>MQGLVVSTHPIYLIAKEITKGVEEPQLLLQGQSGHDVQLTPAHRKAINDASLVIWLGKAHEAPLNKLLSNNKKAIALLDSGILSILPQRNTRGAALPNTVDTHVWLEPNNAVRIGFFIAALRSQQHPENKAKYWNNANTFARNMLQAAQAYDSSSNGKPYWSYHDAYQYLERSLNLKFAGALTDDPHVAPTAAQIKYLNDSRPKAQMCLLAESFTTKGQYQKLGSITF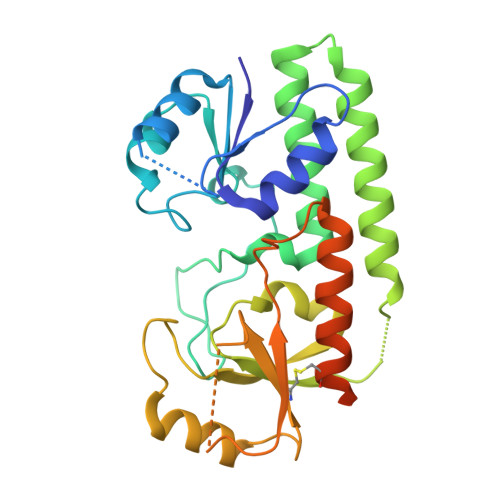QPVDESMNNEDNFVTAWKKLAIKTDKCVLNTQKASLEVLFQGPGSAHHHHHHHHHHHH[2x]Roquins are a family of RNA-binding proteins critically involved in maintaining peripheral immunological tolerance and preventing autoimmune diseases. The human genome encodes two Roquin paralogs, RC3H1 and RC3H2. The N-terminal regions of these two proteins are highly homologous and are composed of a RING (Really Interesting New Gene)-type E3 ubiquitin ligase domain, followed by a unique, so-called ROQ domain of approximately 300 amino acid residues and a CCCH-type ZnF domain5. The ROQ domain binds to a highly conserved, stem-loop-forming constitutive decay element (CDE), which is found in the 3′ UTR of many mRNAs encoding regulators of development and inflammation.

The structure of the RNA-binding region has an elongated shape consisting of 13 α-helices and one β-hairpin. The first three and the last three helices form a tightly packed unit that has little contact with the ROQ domain. This six-helix bundle was found to resemble an HEPN (higher eukaryotes and prokaryotes nucleotide-binding) domain based on a structural homologue search of RC3H1 using DALI9. The HEPN domain of RC3H2 superimposes with that of RC3H1 with a root mean squared deviation (RMSD) of 0.52 Å for all atoms in 145 residues. Analysis using the Rapido algorithm confirmed that this region is composed of two rigid body moieties, which correspond to the HEPN and ROQ domains defined above. The two domains are connected through two flexible, proline-containing (Pro173 and Pro324) linkers and no buried interface exists between them. To compare the inter-domain orientation, we aligned the RC3H2 with the RC3H1 structure against the HEPN domain and found that the ROQ domain of RC3H2 is rotated 34° and shifted 2.5 Å away from the RC3H1 ROQ domain along an axis intersecting the two domains. It is unlikely that this difference is caused by the RING domain in the RC3H1 structure because the RING domain has a large contact area of 863 Å2 with the N-terminal helices of the HEPN domain, but makes no contact with the ROQ domain. The RNA-binding region can be separated into two domains, ROQ and HEPN, which move relatively independently. However, neither our apo-RC3H2 structure nor the RC3H2/RNA complex structure contains a similar protein-protein interface in the crystal packing.

> MSNLGENKHYEVAKKCVEDLALYLKPLSGGKGVASLNQSALSRPMQRKLVTLVNCQLVEEEGRVRAMRAARSLGERTVTELILQHQNPQQLSANLWAAVRARGCQFLGPAMQEEALKLVLLALEDGSALSRKVLVLFVVQRLEPRFPQASKTSIGHVVQLLYRASCFKVTKRDEDSSLMQLKEEFRSYEALRREHDAQIVHIAMEAGLRISPEQWSSLLYGDLAHKSHMQSIIDKLQSPESFAKSVQELTIVLQRTGDPANLNRLRPHLELLANIDPNPDAVSPTWEQLENAMVAVKTVVHGLVDFIQNYSRKGHETPQHHHHHH In an attempt to obtain such “snapshots” of biantennary N-glycan, we selected for crystallographic studies two unrelated plant lectins, Calsepa from Calystegia sepium and PHA-E from Phaseolus vulgaris, which show 4- to 5-fold increase in affinity toward bisected biantennary N-glycans compared with control non-bisected glycan. The most populated conformation of bisected N-glycan is termed the ‘back-fold’ conformation, in which the α1–6 arm is flipped back towards the stem region of N-glycan (GlcNAcβ1–4GlcNAc). In summary, our study provides the first atomic structures of a flipped-back conformation of bisected N-glycan bound to two specific lectins. Thus both proteins, PHA-E as well as Calsepa, are specifically ‘back-fold conformer selective’, rather than broad bisecting GlcNAc-selective lectins.

PHA-E is a legume lectin (120 kDa as tetramer) which is widely used for detecting bisected glycans. Unfortunately, electron density was observed for only two sugar residues from one branch, which made it impossible to decipher the conformation of the whole glycan. We have now determined the crystal structure of PHA-E in complex with a longer bisected N-glycan derivative (glycan 2 in Fig. 4A) at 3.0 Å resolution. Eight PHA-E subunits and eight bisected glycan molecules are packed in the asymmetric unit. PHA-E forms a tetramer and each monomer binds to one bisected glycan in its primary binding site. The structure contains eight carbohydrate residues out of ten. The α1–6 branch and bisecting GlcNAc interact with PHA-E, while the α1–3 branch and chitobiose unit are exposed to solvent. The only hydrogen bonds are between two hydroxyl groups, OH3 and OH4 of GlcNAc-7 and the side chain of Asp122 in the loop B region. The putative H2 and H4 hydrogen atoms of GlcNAc-7 can make van der Waals contact with H1, H3 and H5 hydrogen atoms of GlcNAc-5 of the α1–3 branch. Moreover, the nitrogen atom of GlcNAc-5′ in the α1–6 branch is located within hydrogen bond distance of OH3 of GlcNAc-2 in the chitobiose unit. As in the case of Calsepa, the back-fold conformation appears critical for simultaneous recognition of both the α1–6 branch and GlcNAc-7.

>MASSNLLSLALFLVLLTHANSASQTSFSFQRFNETNLILQRDATVSSKGQLRLTNVNDNGEPTLSSLGRAFYSAPIQIWDNTTGAVASFATSFTFNIDVPNNSGPADGLAFVLLPVGSQPKDKGGLLGLFNNYKYDSNAHTVAVEFDTLYNVHWDPKPRHIGIDVNSIKSIKTTTWDFVKGENAEVLITYDSSTKLLVASLVYPSLKTSFIVSDTVDLKSVLPEWVIVGFTATTGITKGNVETNDILSWSFASKLSDGTTSEALNLANFALNQIL[8x]>MIILAFDIFGTVLDTSTVIQEFRNKQLEYTWLLTIMGKYVEFEEITKITLRYILKVRGEESKFDEELNKWKNLKAYEDTKYLKEISEIAEVYAL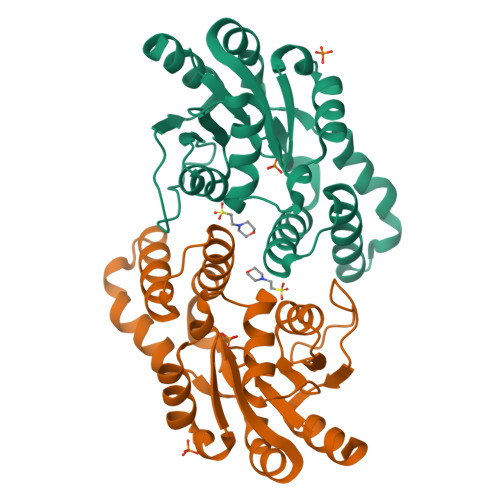SNGSINEVKQHLERNGLLRYFKGIFSAESVKEYKPSPKVYKYFLDSIGAKEAFLVSSNAFDVIGAKNAGMRSIFVNRKNTIVDPIGGKPDVIVNDFKELYEWILRYK[2x]>[5x]FRERLKELVVPKHVMDVVDEELSKLGLLDNHSSEFNVTRNYLDWLTSIPWGKYSNENLDLARAQAVLEEDHYGMEDVKKRILEFIAVSQLRGSTQGKILCFYGPPGVGKTSIARSIARALNREYFRFSVGGMTDVAEIKGHRRTYVGAMPGKIIQCLKKTKTENPLILIDEVDKIGRGYQGDPSSALLELLDPEQNANFLDHYLDVPVDLSKVLFICTANVTDTIPEPLRDRMEMINVSGYVAQEKLAIAERYLVPQARALCGLDESKAKLSSDVLTLLIKQYCRESGVRNLQKQVEKVLRKSAYKIVSGEAESVEVTPENLQDFVGKPVFTVERMYDVTPPGVVMGLAWTAMGGSTLFVETSLRRPQDKDAKGDKDGSLEVTGQLGEVMKESARIAYTFARAFLMQHAPANDYLVTSHIHLHVPEGATPKDGPSAGCTIVTALLSLAMGRPVRQNLAMTGEVSLTGKILPVGGIKEKTIAAKRAGVTCIVLPAENKKDFYDLAAFITEGLEVHFVEHYREIFDIAF

The human mitochondrial AAA+ protein LONP1 is a critical quality control protease involved in regulating diverse aspects of mitochondrial biology including proteostasis, electron transport chain activity, and mitochondrial transcription. The LONP1 protease consists of an N-terminal domain involved in substrate recognition and oligomerization, a AAA+ (ATPases associated with diverse cellular activities) domain that powers substrate translocation, and a C-terminal serine protease domain involved in substrate proteolysis. In mammals, LONP1 is a primary quality control protease responsible for regulating proteostasis and various biological functions within the mitochondrial matrix through diverse mechanisms. Here, we determine structures for human LONP1 in three different states: substrate-free, substrate-bound, and both substrate- and bortezomib-bound.

We show that in the absence of substrate, LONP1 adopts an open, left-handed spiral conformation that is bound to ADP and has its protease active sites organized in an inactive conformation. The substrate-free human LONP1 reconstruction identified in our dataset was resolved to ~3.4 Å resolution, which was sufficient for atomic modeling of five of the six LONP1 protomers. The uppermost subunit of substrate-free human LONP1 hexamer demonstrates substantially more flexibility than its bacterial counterpart, as it is only discernible at low resolution in a subset of the particles. Due to the low resolution of this uppermost subunit, a copy of the middle protomer from the five-subunit spiral was rigid body fit into the low-pass filtered reconstruction for representational purposes. The presence of a fully ADP-bound LONP1 conformation, despite incubating the sample with saturating amounts of ATPγS, likely stems from two factors: the LONP1 sample was purified without supplementing ATP, and the presence of contaminating ADP in the ATPγS stock. According to the previously proposed mechanism of substrate engagement, the topmost subunit of the left-handed spiral is the first to undergo nucleotide exchange upon interaction with substrate, followed by subsequent nucleotide and substrate engagement events that lead to a reorganization of the AAA+ domains within the hexamer into an active state that is competent for substrate translocation. The similarity of the substrate-free human and bacterial structures suggests conservation of this substrate engagement mechanism.> GSDEFTA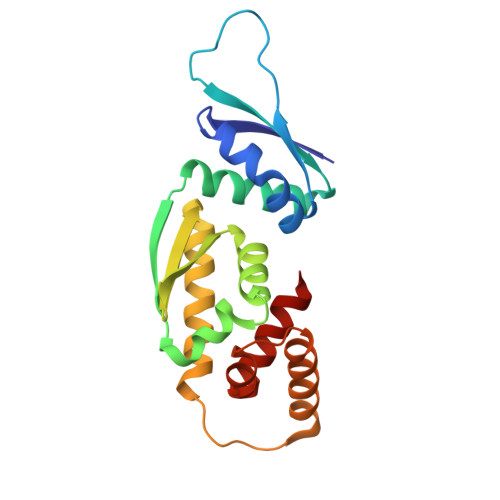PAEKAELLEQSRGRIEGLFGVSLAVLGALGAEEPLPARIWLQLCGAQEAVHSAKEYIKGICEPELEERECYPKDMHCIFVGAESLFLKSLIQDTCADLCILDIGLLGIRGSAEAVVMARSHIQQFVKLFENKENLPSSQKESEVKREFKQFVEAHADNYTMDLLILPTSLKKELLTLTQGE>HPEFLKAGKEPGLQIWRVEKFDLVPVPTNLYGDFFTGDAYVILKTVQLRNGNLQYDLHYWLGNECSQDESGAAAIFTVQLDDYLNGRAVQHREVQGFESATFLGYFKSGLKYKKGGVASGFKHVVPNEVVVQRLFQVKGRRVVRATEVPVSWESFNNGNCFILDLGNNIHQWCGSNSNRYERLKATQVSKGIRDNERSGRARVHVSEEGTEPEAMLQVLGPKPALPAGTEDTAKEDAANRKLAKLYKVSNGAGTMSVSLVADENPFAQGALKSEDCFILDHGKDGKIFVWKGKQANTEERKAALKTASDFITKMD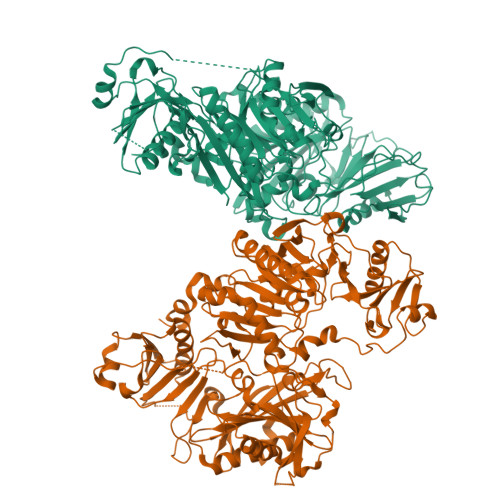YPKQTQVSVLPEGGETPLFKQFFKNWRDPDQTDGLGLSYLSSHIANVERVPFDAATLHTSTAMAAQHGMDDDGTGQKQIWRIEGSNKVPVDPATYGQFYGGDSYIILYNYRHGGRQGQIIYNWQGAQSTQDEVAASAILTAQLDEELGGTPVQSRVVQGKEPAHLMSLFGGKPMIIYKGGTSREGGQTAPASTRLFQVRANSAGATRAVEVLPKAGALNSNDAFVLKTPSAAYLWVGTGASEAEKTGAQELLRVLRAQPVQVAEGSEPDGFWEALGGKAAYRTSPRLKDKKMDAHPPRLFACSNKIGRFVIEEVPGELMQEDLATDDVMLLDTWDQVFVWVGKDSQEEEKTEALTSAKRYIETDPANRDRRTPITVVKQGFEPPSFVGWFLGWDDDYWSVDPLDRAMAELAA[2x]> GTYRKLPLFEGELPEGSYAQIVEVKPKQTVKKHYHERQYELFYIISGEARLGIGD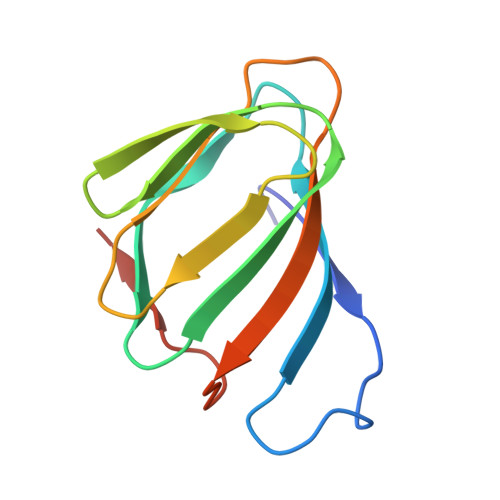TEYQAKPGDIFLVKPKTVHWVVNEKDEPFRLFVVKLNYHGDDSVWLEGSF> MARKYFVAANWKCNGTLESIKSLTNSFNNLDFDPSKLDVVVFPVSVHYDHTRKLLQSKFSTGIQNVSKFGNGSYTGEVSAEIAKDLNIEYVIIGHFERRKYFHETDEDVREKLQASLKNNLKAVVCFGESLEQREQNKTIEVITKQ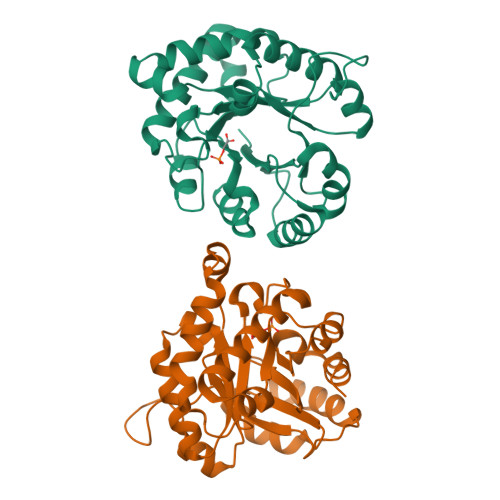VKAFVDLIDNFDNVILVYEPLWAIGTGKTATPEQAQLVHKEIRKIVKDTCGEKQANQIRILYGGSVNTENCSSLIQQEDIDGFLVGNASLKESFVDIIKSAM>[2x]MTLSIPPSIQCQTEAACRLITRVTGDTLRAIHLYGSAVAGGLKPNSDIDLLVTICQPLTEAQRATLMQELLALSSPPGASAEKRALQVTVVLYSQLVPWCFPPSREMQFGEWLREDICQGIYEPAQQDWDMVLLITQILETSIPLKGERAERLFTPAPAAQLLKALRYPLDLWQSTADVQGDEYHIVLTLARIWYTLSTGRFTSKDAAADWLLPQLPEDYAATLRAAQREYLGLEQQDWHILLPAVVRF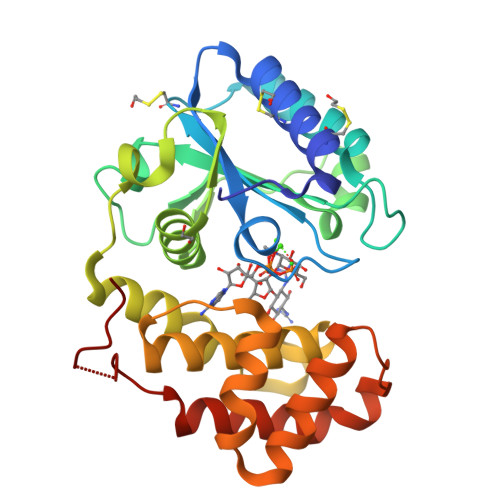VDFAKAHIPTQFTKGHHHHHH> SNAMLRRLFKKKYVCVRQYDLTDCGAA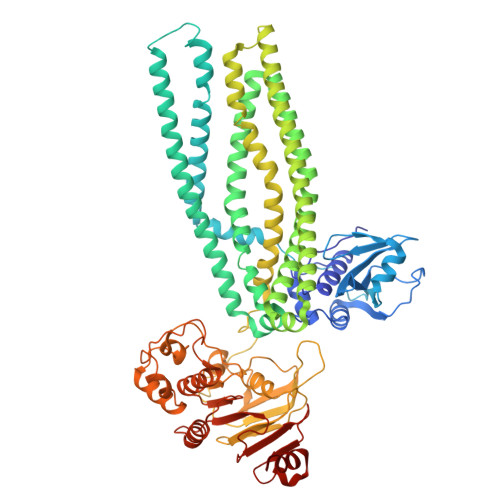CLSSIAQYYGLKMSLAKIREMTGTDTQGTNAYGLIHAAKQLGFSAKGVKASKEDLLKDFRLPAIANVIVDNRLAHFVVIYSIKNRIITVADPGKGIVRYSMDDFCSIWTGGLVLLEPGEAFQKGDYTQNMMVKFAGFLKPLKKTVLCIFLASLLYTALGIAGSFYIKFLFDDLIKFEKLNDLHIISAGFAVIFLLQIFLNYYRSILVTKLGMSIDKSIMMEYYSHVLKLPMNFFNSRKVGEIISRFMDASKIRQAISGATLTIMIDTIMAVIGGILLYIQNSSLFFISFIIILLYGIIVTVFNKPIQNANRQIMEDNAKLTSALVESVKGIETIKSFGAEEQTEKSTRDKIETVMKSSFKEGMLYINLSSLTGIVAGLGGIVILWAGAYNVIKGNMSGGQLLAFNALLAYFLTPVKNLIDLQPLIQTAVVASNRLGEILELATEKELREDSDDFVISLKGDIEFRNVDFRYGLRKPVLKNINLTIPKGKTVAIVGESGSGKTTLAKLLMNFYSPEKGDILINGHSIKNISLELIRKKIAFVSQDVFIFSGTVKENLCLGNENVDMDEIIKAAKMANAHDFIEKLPLKYDTFLNESGANLSEGQKQRLAIARALLKKPDILILDEATSNLDSITENHIKDAIYGLEDDVTVIIIAHRLSTIVNCDKIYLLKDGEIVESGSHTELIALKGCYFKMWKQTENTLAS>[4x]MRIVPFGAAREVTGSAHLLLAGGRRVLLDCGMFQGKEEARNHAPFGFDPKEVDAVLLTHAHLDHVGRLPKLFREGYRGPVYATRATVLLMEIVLEDALKVMDEPFFGPEDVEEALGHLRPLEYGEWLRLGALSLAFGQAGHLPGSAFVVAQGEGRTLVYSGDLGNREKDVLPDPSLPPLADLVLAEGTYGDRPHRPYRETVREFLEILEKTLSQGGKVLIPTFAVERAQEILYVLYTHGH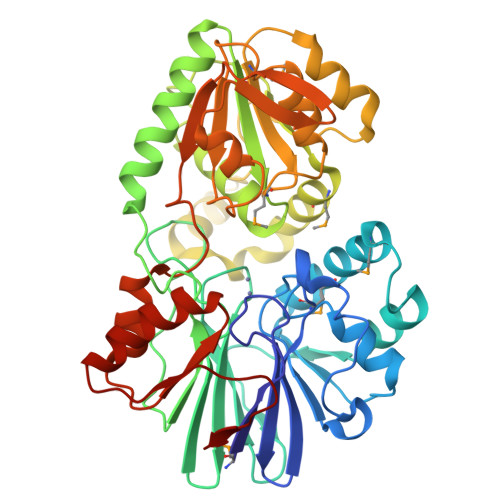RLPRAPIYLDSPMAGRVLSLYPRLVRYFSEEVQAHFLQGKNPFRPAGLEVVEHTEASKALNRAPGPMVVLAGSGMLAGGRILHHLKHGLSDPRNALVFVGYQPQGGLGAEIIARPPAVRILGEEVPLRASVHTLGGFSGHAGQDELLDWLQGEPRVVLVHGEEEKLLALGKLLALRGQEVSLARFGEGVPV>ASMAADTPTACCFSYTSRQIPQNFIADYFETSSQCSKPGVIFLTKRSRQVCADPSEEWVQKYMSDLELSA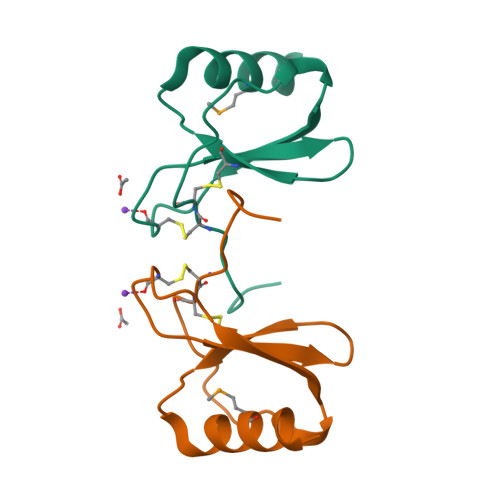[5x]>MSLDIQSLDIQCEELSDARWAELLPLLQQCQVVRLDDCGLTEARCKDISSALRVNPALAELNLRSNELGDVGVHCVLQGLQTPSCKIQKLSLQNCCLTGAGCGVLSSTLRTLPTLQELHLSDNLLGDAGLQLLCEGLLDPQCRLEKLQLEYCSLSAASCEPLASVLRAKPDFKELTVSNNDINEAGVRVLCQGLKDSPCQLEALKLESCGVTSDNCRDLCGIVASKASLRELALGSNKLGDVGMAELCPGLLHPSSRLRTLWIWECGITAKGCGDLCRVLRAKESLKELSLAGNELGDEGARLLCETLLEPGCQLESLWVKSCSFTAACCSHFSSVLAQNRFLLELQISNNRLEDAGVRELCQGLGQPGSVLRVLWLADCDVSDSSCSSLAATLLANHSLRELDLSNNCLGDAGILQLVESVRQPGCLLEQLVLYDIYWSEEMEDRLQALEKDKPSLRVIS[2x];>[2x]MKESRAKKFQRQHMDSDSSPSSSSTYCNQMMRRRNMTQGRCKPVNTFVHEPLVDVQNVCFQEKVTCKNGQGNCYKSNSSMHITDCRLTN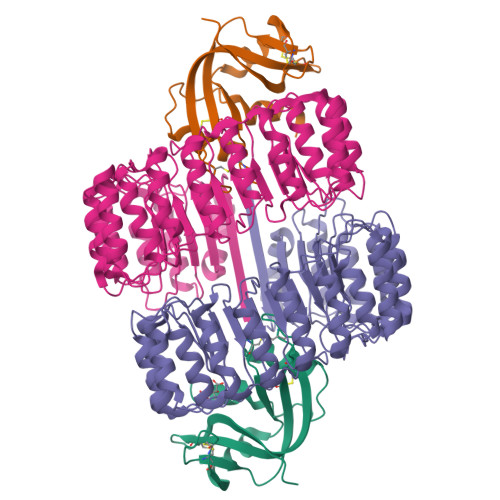GSRYPNCAYRTSPKERHIIVACEGSPYVPVHFDASVEDST> GGSAATWTSLGLTSLGAVSMTTTTEQSFTLPVAAQTASQILVYLRCHSGNASTTGADDIRIYTKEGAATYDHYLLMFPYAGQGAVGYNSDSFWLPKTSDNKIYLAHSMAPGSANSGCNFYITGYK

Bdellovibrio bacteriovorus is a bacterium that preys upon a wide range of other Gram-negative bacteria, entering their periplasm and consuming them from within. Proteomic and structural analyses of vesicle contents reveal several fibre-like proteins, which we name the mosaic adhesive trimer (MAT) superfamily, and show localization on the predator surface before prey encounter. Structural studies reveal a variety of domain usages (and therefore binding capabilities) at the fibre C-termini, placing these on intertwined trimeric β-prisms. Using independent but complementary approaches, we identified and characterized a MAT superfamily of trimeric fibre proteins with diverse adhesive tips, able to fulfil the long-sought-after role of multiplicity of molecular recognition and handling of diverse epitopes (across a wide prey range), by the bacterial predator B. bacteriovorus.

The β-sandwich tip domain of Bd2133 adopts a twisted fold, trimerizing about strand G989–W999 (burying 5,640 Å2 per monomer). There are several atoms lying on the three-fold axis. Solving a 1 Å tip-only variant (A910 onwards) allowed us to confidently model these as a water, a sodium and a chloride ion. Unexpectedly, there are no homologues of this domain in the PDB (judged by DALI16), but FoldSeek19 found strong homology to Synechococcaceae and Competibacter proteins.> GP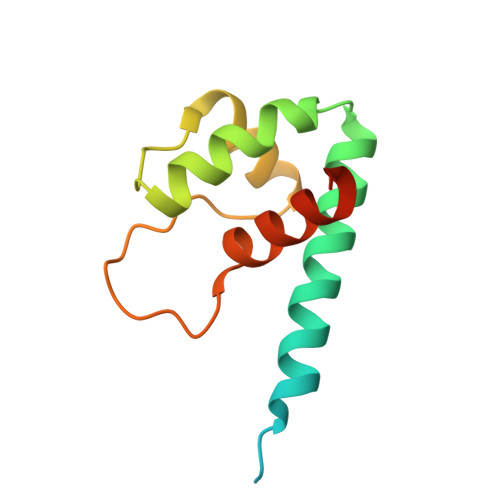LGSDRASQTPVDRSPPRVNQRPIRVDRAAMRNRGNDEADAALRGLVQQGVNLEHLRTALERHVMQRLPIPLDIGSALQNVGINPSIDLGESLVQHPLLNLNVALNRMLGLRPSAE> MHNHNHN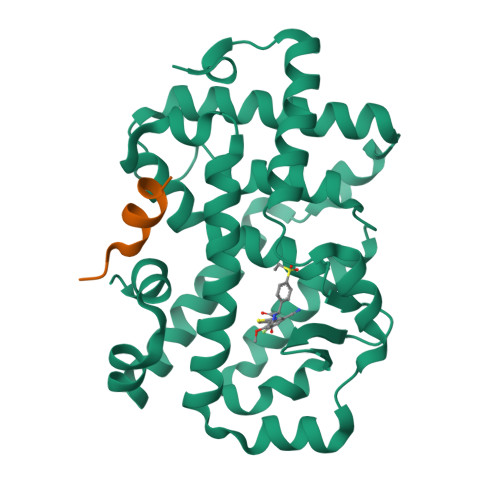HNHNHNGGENLYFQGASLTEIEHLVQSVCKSYRETCQLRLEDLLRQRSNIFSREEVTGYQRKSMWEMWERCAHHLTEAIQYVVEFAKRLSGFMELCQNDQIVLLKAGAMEVVLVRMCRAYNADNRTVFFEGKYGGMELFRALGCSELISSIFDFSHSLSALHFSEDEIALYTALVLINAHRPGLQEKRKVEQLQYNLELAFHHHLCKTHRQSILAKLPPKGKLRSLCSQHVERLQIFQHLHPIVVQAAFPPLYKELFSGG;> KHKILHRLLQDS>GSHMLPDPNGCLTAAGAFSSDERAAVYRAIETRRDVRDEFLPEPLSEELIARLLGAAHQAPSVGFMQPWNFVLVRQDETREKVWQAFQRANDEAAEMFSGERQAKYRSLKLEGIRKAPLSICVTCDRTRGGAVVLGRTHNPQMDLYSTVCAVQNLWLAARAEGVGVGW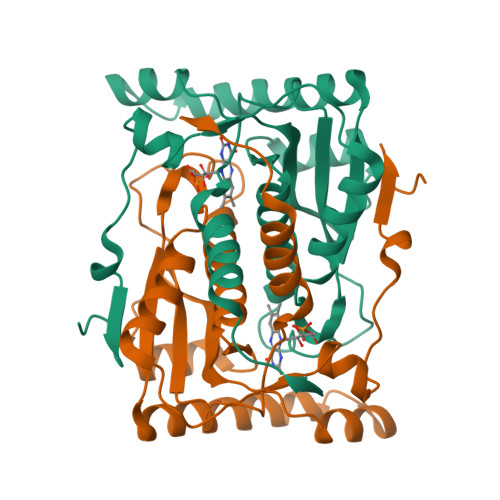VSIFHESEIKAILGIPDHVEIVAWLCLGFVDRLYQEPELAAKGWRQRLPLEDLVFEEGWGVR[8x]>[2x]MAEKPKLHYFNARGRMESTRWLLAAAGVEFEEKFIKSAEDL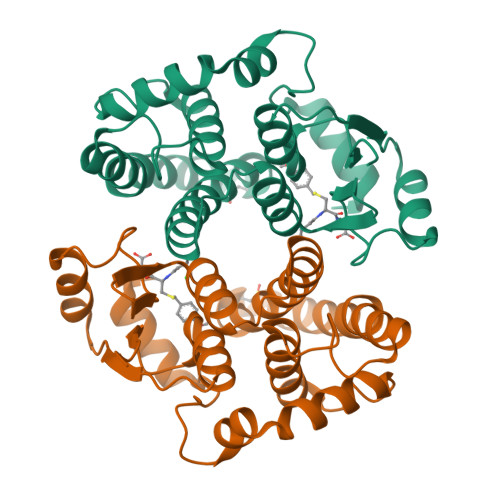DKLRNDGYLMFQQVPMVEIDGMKLVQERAILNYIASKYNLYGKDIKERALIDMYIEGIADLGEMILLLPVCPPEEKDAKLALIKEKIKNRYFPAFEKVLKSHGQDYLVGNKLSRADIHLVELLYYVEELDSSLISSFPLLKALKTRISNLPTVKKFLQPGSPRKPPMDEKSLEEARKIFRF> MVQQLSLFGSIGDDGYDLLISTLTTISGNPPLLYNSLCTVWKPNPSYDVENVNSRNQLVEPNRIKLSKEVPFSYLIDETMMDKPLNFRILKSFTNDKIPLNYAMTRNINSDDIIDVDMDASPAPSNESCSPWS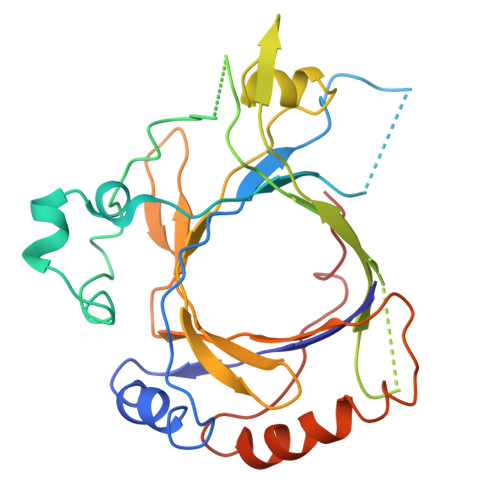LQISDIPAAGNNRSVSMQTIAETIILSSAGKNSSVSSLMNGLGYVFEFQYLTIGVKFFMKHGLILELQKIWQIEEAGNSQITSGGFLLKAYINVSRGTDIDRINYTETALMNLKKELQGYIELSVPDRQSMDSRVAHGNILI The endoplasmic-reticulum aminopeptidase ERAP1 processes antigenic peptides for loading on MHC-I proteins and recognition by CD8 T cells as they survey the body for infection and malignancy. ERAP1 is a member of the M1 aminopeptidase family, which is found in all domains of life and plays numerous functional roles. These proteins contain a thermolysin-like domain10 (domain II), which holds the active site. The M1 aminopeptidase family has a conserved HEAT-motif-repeat domain (domain IV) forming a bowl-shaped C-terminal structure.

To examine the effect of active-site occupancy on ERAP1 conformation in solution, we used a tight-binding tripeptide analog DG013 (IC50 = 33 nM29), which has a phosphinic group expected to mimic the tetrahedral intermediate that would form at the scissile peptide bond during catalysis. We determined the X-ray crystal structure of ERAP1 bound to DG013 (see “Methods” for details) and confirmed that DG013 binds as expected to the ERAP1 active site, with the enzyme adopting the closed conformation in the crystal. The binding pose is similar to that of another phosphinic peptide, DG046, bound to ERAP130, but distinct from DG013 bound to ERAP2, most likely due to lack of an aromatic P2’-binding site. In the presence of DG013, ERAP1 Rg decreases by ~2 Å, an effect observed in multiple measurements and for two independent protein preparations (yellow circles). Fitting the ERAP1 + DG013 scattering profiles to molecular dynamics structures revealed a cluster of models consistent with the experimental data (Χ2 < 1) with theta between 54 and 62° (yellow symbols). This cluster is distinct and nonoverlapping with that observed for ERAP1 in the absence of DG013, and consistent with a conformation similar to but slightly more open than observed for ERAP1 in closed-conformation crystal structures. In the ERAP1–DG014 (open) complex, (cyan) as in previous open ERAP1 crystal structures, Tyr438 is oriented away from the active site and moves to interact with the peptide bond transition-state mimic phosphinic group in the ERAP1-DG013 (closed) complex (magenta), in a position analogous to the previously determined bestatin-bound ERAP1 closed structure. Reorientation of Phe433 and motion of the helix 4a is coupled to rotation and tilt of helix 5, which repositions the side chain of Tyr438.

>QSTEASPKRHHHHHHHHHHSDENLYFQGTPFPWNKIRLPEYVIPVHYDLLIHANLTTLTFWGTTKVEITASQPTSTIILHSHHLQISRATLRKGAGERLSEEPLQVLEHPRQEQIALLAPEPLLVGLPYTVVIHYAGNLSETFHGFYKSTYRTKEGELRILASTQFEPTAARMAFPCFDEPAFKASFSIKIRREPRHLAISNMPLVKSVTVAEGLIEDHFDVTVKMSTYLVAFIISDFESVSKITKSGVKVSVYAVPDKINQADYALDAAVTLLEFYEDYFSIPYPLPKQDLAAIPDFQSGAMENWGLTTYRESALLFDAEKSSASSKLGITMTVAHELAHQWFGNLVTMEWWNDLWLNEGFAKFMEFVSVSVTHPELKVGDYFFGKCFDAMEVDALNSSHPVSTPVENPAQIREMFDDVSYDKGACILNMLREYLSADAFKSGIVQYLQKHSYKNTKNEDLWDSMASIGGGGVDVKTMMNTWTLQKGFPLITITVRGRNVHMKQEHYMKGSDGAPDTGYLWHVPLTFITSKSDMVHRFLLKTKTDVLILPEEVEWIKFNVGMNGYYIVHYEDDGWDSLTGLLKGTHTAVSSNDRASLINNAFQLVSIGKLSIEKALDLSLYLKHETEIMPVFQGLNELIPMYKLMEKRDMNEVETQFKAFLIRLLRDLIDKQTWTDEGSVSERMLRSQLLLLACVHNYQPCVQRAEGYFRKWKESNGNLSLPVDVTLAVFAVGAQSTEGWDFLYSKYQFSLSSTEKSQIEFALCRTQNKEKLQWLLDESFKGDKIKTQEFPQILTLIGRNPVGYPLAWQFLRKNWNKLVQKFELGSSSIAHMVMGTTNQFSTRTRLEEVKGFFSSLKENGSQLRCVQQTIETIEENIGWMDKNFDKIRVWLQSEKLER[22x]The degradation of HIFα subunits is promoted by post-translational hydroxylation of prolyl-residues located in its N/C-terminal oxygen dependent degradation domains (NODD and CODD). These dioxygen-sensitive reactions are catalysed by 2-oxoglutarate (2OG) and Fe(II) dependent prolyl hydroxylases (PHD 1–3 in humans). The human PHDs catalyse hydroxylation of prolyl-residues within the N/C terminal ODDs of HIF-1/2/3α and are negative regulators of the transcriptionally regulated hypoxic response.

We successfully crystallized cPHD2 in the presence of a 14-residue NCCP (3C), obtained in a RaPID with five rounds of screening. Consistent with the reported NMR studies, we obtained multiple crystal structures revealing that 3C binds in the region of cPHD2 immediately to the N-terminal side of the core distorted double stranded β-helix (DSBH) fold of PHD2. Interestingly, within the crystal lattice, 3C ‘slots’ into a tight groove between the non-DSBH β1 of one cPHD2 molecule and the C-terminal α4 (that is also involved in the P63 crystal packing) of a neighbouring symmetry related cPHD2 molecule. In the cPHD2.3C complex structures, 3C adopts a rectangular fold comprising two (almost) planar distorted β-strands connected by two type II beta turns with DY1, D6, W8 and T13 at its four corners; most of the side chains do not protrude extensively. 3C forms extensive backbone-to-backbone interactions with cPHD2 β1 (aa 204–214) and three residues located at the N-terminus (187–189) within the same cPHD2 monomer and six residues (399–404) located at the C-terminus of a symmetry related cPHD2 molecule.

> GSHMASPNGQTKPLPALKLALEYIVPCMNKHGICVVDDFLGKETGQQIGDEVRALHDTGKFTDGQLVSQKSDSSKDIRGDKITWIEGKEPGCETIGLLMSSMDDLIRHCNGKLGSYKINGRTKAMVACYPGNGTGYVRHVDNPNGDGRCVTCIYYLNKDWDAKVSGGILRIFPEGKAQFADIEPKFDRLLFFWSDRRNPHEVQPAYATRYAITVWYFDADERARAKVKYLTGE;> XYVWLTDTWVLSRT> HPETLVKVKDAEDQ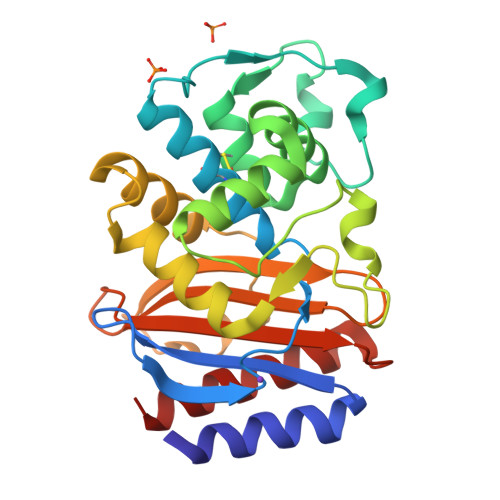LGARVGYIELDLNSGKILESFRPEERFPMVSTFKVLLCGAVLSRVDAGQEQLGRRIHYSQNDLVEYSPVTEKHLTDGMTVRELCSAAITMSDNTAANLLLTTIGGPKELTAFLHNMGDHVTRLDRWEPELNEAIPNDERDTTMPAAMATTLRKLLTGELLTLASRQQLIDWMEADKVAGPLLRSALPAGWFIADKSGAGERGSRGIIAALGPDGKPSRIVVIYTTGSQATMDERNRQIAEIGASLIKHW> MEIPVIEPLFTKVTEDIPGAQGPVFDKNGDFYIVAPEVEVNGKPAGEILRIDLKTGKKTVICKPEVNGYGGIPAGCQCDRDANQLFVADMRLGLLVVQTDGTFEEIAKKDSEGRRMQGCDDCAFDYEGNLWITAPAGEVAPADYTRSMQEKFGSIYCFTTDGQMIQVDTAFQFPDGIAVRHMNDGRPYQLIVAETPTKKLWSYDIKGPAKIENKKVWGHIPGTHEGGANGMDFDEDNNLLVANWGSSHIEVFGPDGGQPKMRIRCPFEKPSNLHFKPQTKTIFV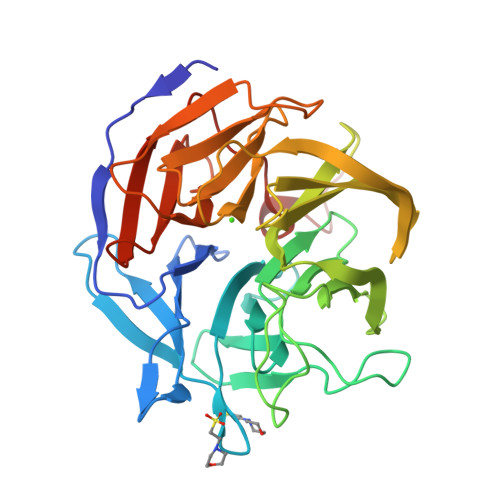TEHENNAVWKFEWQRNGKKQYCETLKFGIF>MGKRAAHIGLRALADLATPMAVRVAATLRVADHIAAGHRTAAEIASAAGAHADSLDRLLRHLVAVGLFTRDGQGVYGLTEFGEQLRDDHAAGKRKWLDMNSAVGRGDLGFVELAHSIRTGQPAYPVRYGTSFWEDLGSDPVLSASFDTLMSHHLELDYTGIAAKYDWAALGHVVDVGGGSGGLLSALLTAHEDLSGTVLDLQGPASAAHRRFLDTGLSGRAQVVVGSFFDPLPAGAGGYVLSAVLHDWDDLSAVAILRRCAEAAGSGGVVLVIEAVAGDEHAGTGMDLRML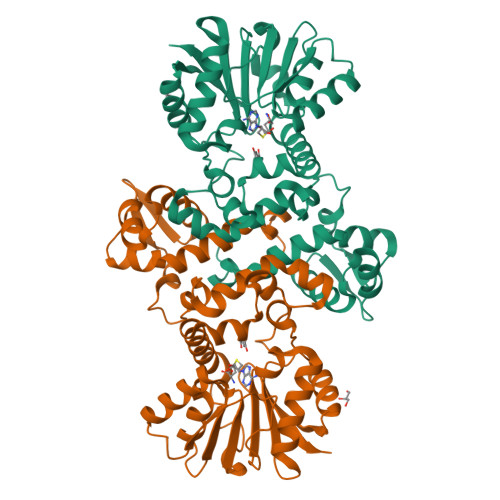TYFGGKERSLAELGELAAQAGLAVRAAHPISYVSIVEMTAL[2x]>[4x]SMVMKKSKTIGVIVPDITNPFFAQLIRGIESVLYKENFILILCNADQDVTREHEYLTELIRRSVDGFVIASSEISNQTINETLRAKKIPFIVLDQKKAEGFSDAVLTDDYRGGQLAAKHLQEQRHEQVIVVMPPHAPVNIQQRLKGFCSVYTEKVQLIETELSKTGGYQAVPEILKTESTGIFAINDEIAFGLYRG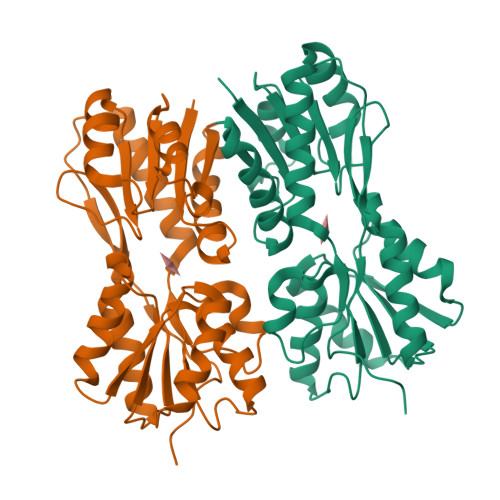LAEAGKKIPEDYSIIGYDNVDMCEYVSPPLTTIAQPVFQLGQTTATLLLERIHQPAKDWEEQTLPVQLIERFSTAPLK>[2x]CCGGACGAGGUGCGCCGUACCCGGUCAGGACAAGACGGCGC

We have determined high-resolution crystal structures of the ykkC guanidine III riboswitch from Thermobifida fusca. X-ray crystallography shows that the RNA folds into an H-type pseudoknot, in which a connecting strand locates in the major groove of one duplex to form a regular triple helix. This continues into the central core of conserved nucleotides that form a novel left-handed helical ramp of inter-nucleotide interactions, generating the guanidinium cation binding site. Comparison with earlier probing data suggest that the formation of the triple helix is stabilized by guanidine binding and this exposes the adjacent ribosome binding site to permit initiation of gene translation.

In this work we have crystallized the guanidine III riboswitch and solved its structure by X-ray crystallography at a resolution of 1.91 Å. The helical ramp creates the guanidine binding site of the riboswitch. Two of the guanidino nitrogen atoms are hydrogen bonded to O6 and N7 on the Hoogsteen edge of G7, while two are equivalently bonded to G17, so that one ligand nitrogen is hydrogen bonded to the O6 atoms of both G7 and G17 nucleobases. Hydrogen bonding between guanidine and the Hoogsteen edge of guanine also occurs in guanidine riboswitches I (Battaglia et al., 2017, Reiss et al., 2017) and II (Huang et al., 2017), but this is the first case where the ligand is simultaneously bonded to two guanine nucleobases in this same manner. The nitrogen atom that is bonded to N7 of G7 is also hydrogen bonded to the O2′ of the ribose of C6, but the nitrogen atom bonded to N7 of G17 only makes the one interaction with the RNA. Thus while five of the six guanidino protons are hydrogen bonded to RNA ligands, the sixth is not. However the experimental phasing map shows clear density in the position that would be occupied by a sixth acceptor, which we tentatively assign as a water molecule. Lastly, we observe that the guanidine is stacked on the nucleobase of C6 at a distance of 3.5 Å. This is a π-cation interaction (Gallivan and Dougherty, 1999, Wintjens et al., 2000) between the positively charged guanidino cation and the aromatic nucleobase. Examination of a space-filling representation of the guanidine III riboswitch structure shows that there is an opening in the side facing the proton that is unbonded to RNA.> MVSFRLSGATSSSYGVFISNLRKALPNERKLYDIPLLRS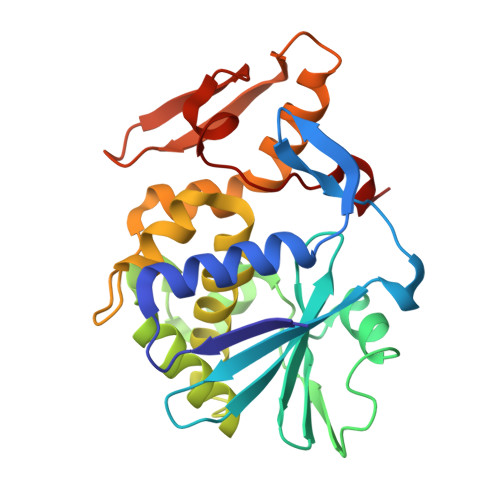SLPGSQRYALIHLTNYADETISVAIDVTNVYIMGYRAGDTSYFFNEASATEAAKYVFKDAMRKVTLPYSGNYERLQTAAGKIRENIPLGLPALDSAITTLFYYNANSAASALMVLIQSTSEAARYKFIEQQIGKRVDKTFLPSLAIISLENSWSALSKQIQIASTNNGQFESPVVLINAQNQRVTITNVDAGVVTSNIALLLNRNNMA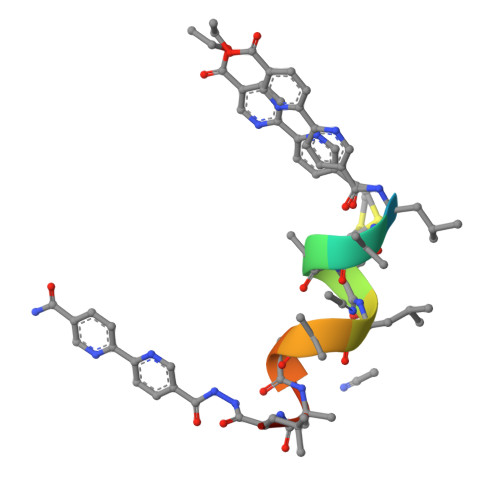> XLAAMLAQALX>[2x]DTYTWKNARIDGGGFVPGIVFNRSEKNLAYARTDIGGAYRWDQSGKQWKPLLDWVDWDRWGWTGVVSLASDTVDPDNVYAAVGTYTNSWDPTDGAVLRSSDRGASWKAATLPFKLGGNMPGRGMGERLAVDPNKNSVLYLGAPSGNGLWRSTDAGVSWSEVTAFPNPGNYAQDPSDTSGYG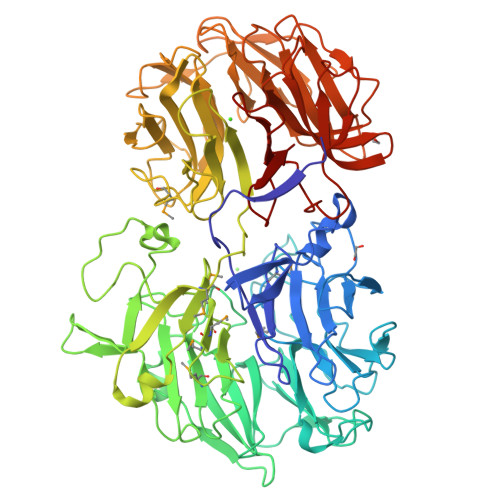NDNQGIVWVTFDERSGSAGSATQDIYVGVADKENTVYRSTDGGATWSRIPGQPTGYLAHKGVLDSATGHLYLTLSDTGGPYDGGKGRIWRYDTASGAWQDVSPVAEADAYYGFSGLSVDRQKPGTLMATAYSSWWPDTQIFRSTDSGATWTQAWDYTGYPNRSNRYTLDVSSVPWLSWGASPAPPETAPKLGWMTEALEIDPFDSDRMMYGTGATVYGTEDLTSWDSGGTFRITPMVKGIEETAVNDLASPPSGAPLLSALGDIGGFRHTDLDAVPDLMYTSPNLDSTTSLDFAESSPGTVVRVGNSDAAPHIGFSTDNGANWFQGSEPSGVTGGGTVAAAADGSGFVWSPEGAGVHHTTGFGTSWTASTGIPAGATVESDRKNPEKFYGFEAGTFYVSTDGGATFTAEATGLPAEGNVRFQALPGTEGDIWLAGGSDTGAYGLWRSTDSGATFTKSAGVEQADSVGFGKAAPGASYRTVFVSAKIGGVRGIFRSTDAGASWTRINDDAHQWGWTGAAITGDPRVYGRVYVSTNGRGIQVGET N-[8-(1,2,3,4-TETRAHYDROACRIDIN-9-YLTHIO)OCTYL]-1,2,3,4-TETRAHYDROACRIDIN-9-AMINE 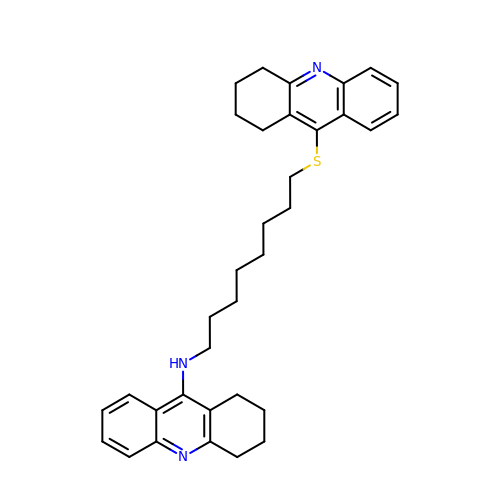| C34 H41 N3 S | COEYCPFFRLYNSC-UHFFFAOYSA-N6-(2-fluoro-6-methoxyphenyl)-1-[4-(4-methylpiperazin-1-yl)phenyl]-1H-pyrazolo[4,3-c]pyridine | C24 H24 F N5 O | 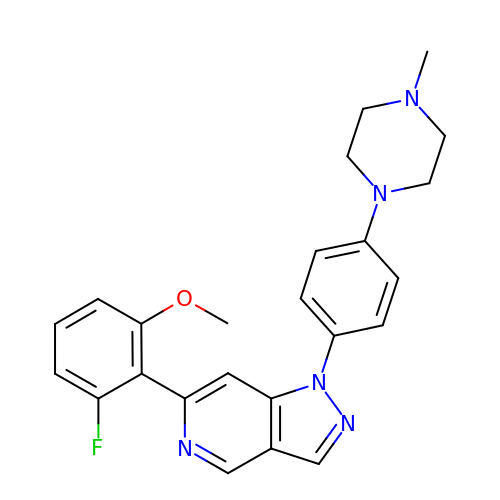AKYAXKVIYVHHNH-UHFFFAOYSA-N>IRAQASAVEAPATAKAKKESKKQEEGVVTNLYKPKEPYVGRCLLNTKITGDDAPGETWHMVFSTEGKIPYREGQSIGVIADGVDKNGKPHKVRLYSIASSAIGDFGDSKTVSLCVKRLIYTNDAGEIVKGVCSNFLCDLQPGDNVQITGPVGKEMLMPKDPNATIIMLATGTGIAPFRSFLWKMFFEKHDDYKFNGLGWLFLGVPTSSSLLYKEEFGKMKERAPENFRVDYAVSREQTNAAGERMYIQTRMAEYKEEL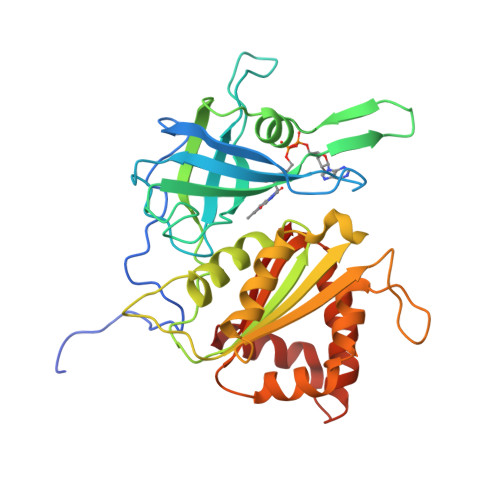WELLKKDNTYVYMCGLKGMEKGIDDIMVSLAEKDGIDWFDYKKQLKRGDQWNVEVY[2x]> PEIVDTCSLASPASVCRTKHLHLRCSVDFTRRTLTGTAALTVQSQEDNLRSLVLDTKDLTIEKVVINGQEVKYALGERQSYKGSPMEISLPIALSKNQEIVIEISFETSPKSSALQWLTPEQTSGKEHPYLFSQCQAIHCRAILPCQDTPSVKLTYTAEVSVPKELVALMSAIRDGETPDPEDPSRKIYKFIQKVPIPCYLIALVVGALESRQIGPRTLVWSEKEQVEKSAYEFSETESMLKIAEDLGGPYVWGQYDLLVLPPSFPYGGMENPCLTFVTPTLLAGDKSLSNVIAHEISHSWTGNLVTNKTWDHFWLNEGHTVYLERHICGRLFGEKFRHFNALGGWGELQNSVKTFGETHPFTKLVVDLTDIDPDVAYSSVPYEKGFA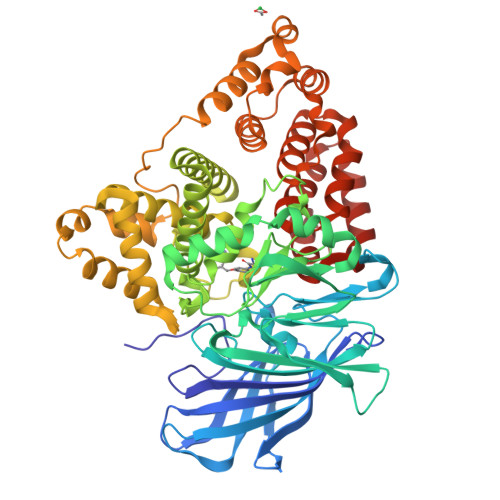LLFYLEQLLGGPEIFLGFLKAYVEKFSYKSITTDDWKDFLYSYFKDKVDVLNQVDWNAWLYSPGLPPIKPNYDMTLTNACIALSQRWITAKEDDLNSFNATDLKDLSSHQLNEFLAQTLQRAPLPLGHIKRMQEVYNFNAINNSEIRFRWLRLCIQSKWEDAIPLALKMATEQGRMKFTRPLFKDLAAFDKSHDQAVRTYQEHKASMHPVTAMLVGKDLKVD>WNSRYSYNQLKNKDSLIMFLVEIFRSLFVSNCIDKNIDNVLLSIEEMFIDHYYNPQHSRLKYLIDDVGIFFTKLPITKAFHTYNKKYRITKRLYAPPTFNEVRHILNLAQILSLEEGLDLLTFDANETLYPDGHDFNDEVLASYISCLLKKMNIAIVTAASYNNDAEKYQKRLENLLKYFSKHNIKDGSYKNFYVMGGESNYLFKCNEEATLYSVPENEWRHYKKFVDYDTVQEILNISEKCLEKVIKDFGLCAQIQRKEKSIGLVPNKIPSLNIKNEQKNYMIKYEVLEEAVIRIKKEIIKNKITAPYCAFNGGQDLWVDVGNKAEGLLILQKLLKIQKKKCCHIGDQFLHSGNDFPTRFCSLTLWVSNPQETKACLKSIMHL[2x];>[2x]QWNSRYSYNQLKNKDSLIMFLVEIFRSLFVSNCIDKNIDNVLLSIEEMFIDHYYNPQHSRLKYLIDDVGIFFTKLPITKAFHTYNKKYRITKRLYAPPTFNEVRHILNLAQILSLEEGLDLLTFDANETLYPDGHDFNDEVLASYISCLLKKMNIAIVTAASYNNDAEKYQKRLENLLKYFSKHNIKDGSYKNFYVMGGESNYLFKCNEEATLYSVPENEWRHYKKFVDYDTVQEILNISEKCLEKVIKDFGLCAQIQRKEKSIGLVPNKIPSLNIKNEQKNYMIKYEVLEEAVIRIKKEIIKNKITAPYCAFNGGQDLWVDVGNKAEGLLILQKLLKIQKKKCCHIGDQFLHSGNDFPTRFCSLTLWVSNPQETKACLKSIMHL;> SDMKKNIVQWNSRYSYNQLKNKDSLIMFLVEIFRSLFVSNCIDKNIDNVLLSIEEMFIDHYYNPQHSRLKYLIDDVGIFFTKLPITKAFHTYNKKYRITKRLYAPPTFNEVRHILNLAQILSLEEGLDLLTFDANETLYPDGHDFNDEVLASYISCLLKKMNIAIVTAASYNNDAEKYQKRLENLLKYFSKHNIKDGSYKNFYVMGGESNYLFKCNEEATLYSVPENEWRHYKKFVDYDTVQEILNISEKCLEKVIKDFGLCAQIQRKEKSIGLVPNKIPSLNIKNEQKNYMIKYEVLEEAVIRIKKEIIKNKITAPYCAFNGGQDLWVDVGNKAEGLLILQKLLKIQKKKCCHIGDQFLHSGNDFPTRFCSLTLWVSNPQETKACLKSIMHLN;>[2x]QWNSRYSYNQLKNKDSLIMFLVEIFRSLFVSNCIDKNIDNVLLSIEEMFIDHYYNPQHSRLKYLIDDVGIFFTKLPITKAFHTYNKKYRITKRLYAPPTFNEVRHILNLAQILSLEEGLDLLTFDANETLYPDGHDFNDEVLASYISCLLKKMNIAIVTAASYNNDAEKYQKRLENLLKYFSKHNIKDGSYKNFYVMGGESNYLFKCNEEATLYSVPENEWRHYKKFVDYDTVQEILNISEKCLEKVIKDFGLCAQIQRKEKSIGLVPNKIPSLNIKNEQKNYMIKYEVLEEAVIRIKKEIIKNKITAPYCAFNGGQDLWVDVGNKAEGLLILQKLLKIQKKKCCHIGDQFLHSGNDFPTRFCSLTLWVSNPQETKACLKSIMHLN;> FVQWNSRYSYNQLKNKDSLIMFLVEIFRSLFVSNCIDKNIDNVLLSIEEMFIDHYYNPQHSRLKYLIDDVGIFFTKLPITKAFHTYNKKYRITKRLYAPPTFNEVRHILNLAQ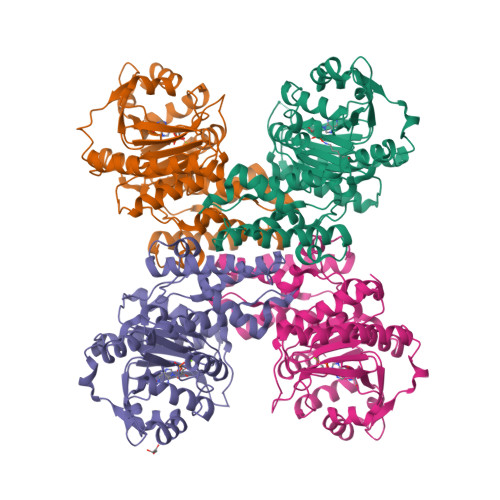ILSLEEGLDLLTFDANETLYPDGHDFNDEVLASYISCLLKKMNIAIVTAASYNNDAEKYQKRLENLLKYFSKHNIKDGSYKNFYVMGGESNYLFKCNEEATLYSVPENEWRHYKKFVDYDTVQEILNISEKCLEKVIKDFGLCAQIQRKEKSIGLVPNKIPSLNIKNEQKNYMIKYEVLEEAVIRIKKEIIKNKITAPYCAFNGGQDLWVDVGNKAEGLLILQKLLKIQKKKCCHIGDQFLHSGNDFPTRFCSLTLWVSNPQETKACLKSIMHLN> GMNTFKTIEELATYIEEQQLVLLFIKTENCGVCDVMLRKVNYVLENYNYVEKIE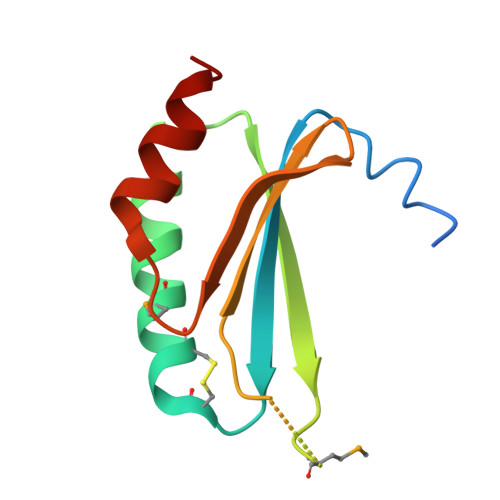ILLQDMQEIAGRYAVFTGPTVLLFYNGKEILRESRFISLENLERTIQLFEE4-O-beta-D-glucopyranosyl-D-gluconic 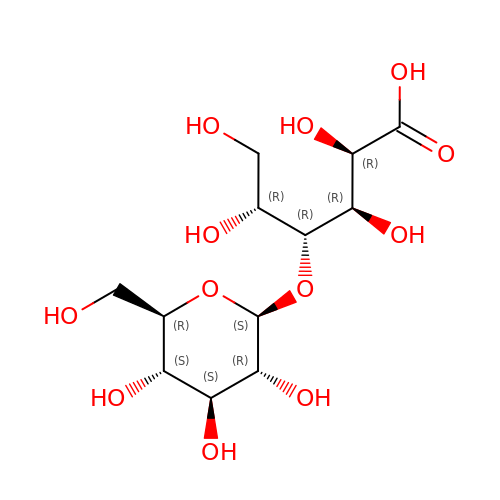acid | C12 H22 O12 | JYTUSYBCFIZPBE-ZNLUKOTNSA-N>MDSKGSSQKGSRLLLLLVVSNLLLCQGVVSGSLQPLPPTAFTPNGTYLQHLARDPTSGTLYLGA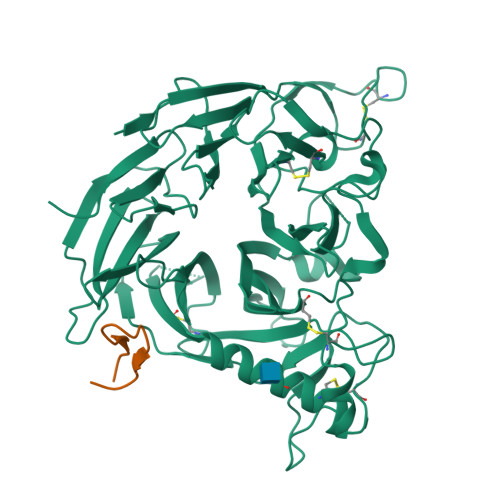TNFLFQLSPGLQLEATVSTGPVLDSRDCLPPVMPDECPQAQPTNNPNQLLLVSPGALVVCGSVHQGVCEQRRLGQLEQLLLRPERPGDTQYVAANDPAVSTVGLVAQGLAGEPLLFVGRGYTSRGVGGGIPPITTRALWPPDPQAAFSYEETAKLAVGRLSEYSHHFVSAFARGASAYFLFLRRDLQAQSRAFRAYVSRVCLRDQHYYSYVELPLACEGGRYGLIQAAAVATSREVAHGEVLFAAFSSAAPPTVGRPPSAAAGASGASALCAFPLDEVDRLANRTRDACYTREGRAEDGTEVAYIEYDVNSDCAQLPVDTLDAYPCGSDHTPSPMASRVPLEATPILEWPGIQLTAVAVTMEDGHTIAFLGDSQGQLHRVYLGPGSDGHPYSTQSIQQGSAVSRDLTFDGTFEHLYVMTQSTLLKVPVASCAQHLDCASCLAHRDPYCGWCVLLGRCSRRSECSRGQGPEQWLWSFQPELGCLQTRENLYFQGKDGGGGGSHMGVAMPGAEDDVV[6x];>XWRPRVARWTGQIIYCSX[6x]> ARKSA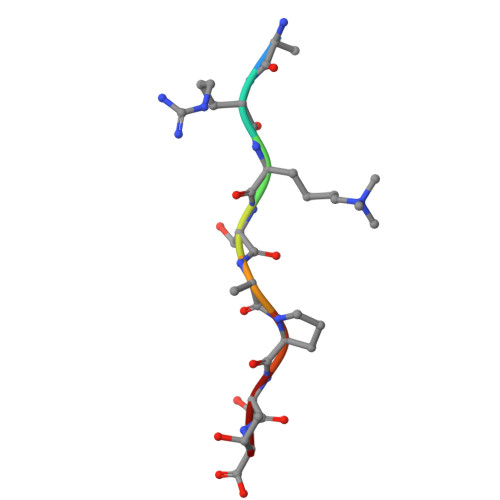PTT> MSSFKYKNSAAGASMQSAANITLRQILEPNNVNLRSKKTHIVCTLGPACKSVETLVKLIDAGMDICRFNFSHGSHEDHKEMFNNVLKAQELRPNCLLGMLLDTKGPEIRTGFLKNKEVHLKEGSKLKLVTDYEFLGDETCIACSYKKLPQSVKPGNIILIADGSVSCKVLETHEDHVITEVLNSAVIGERKNMNLPNVKVDLPIISEKDKNDILNFAIPMGCNFIAASFIQSADDVRLIRNLLGPRGRHIKIIPKIENIEGIIHFDKILAESDGIMIARGDLGMEISPEKVFLAQKLMISKCNLQGKPIITATQMLESMTKNPRPTRAEVTDVANAVLDGTDCVMLSGETAGGKFPVEAVTIMSKICLEAEACIDYKLLYQSLVNAIETPISVQEAVARSAVETAESIQASLIIALTETGYTARLIAKYKPSCTILALSASDSTVKCLNVHRGVTCIKVGSFQGTDIVIRNAIEIAKQRNMAKVGDSVIAIHGIKEEVSGGTNLMKVVQIEL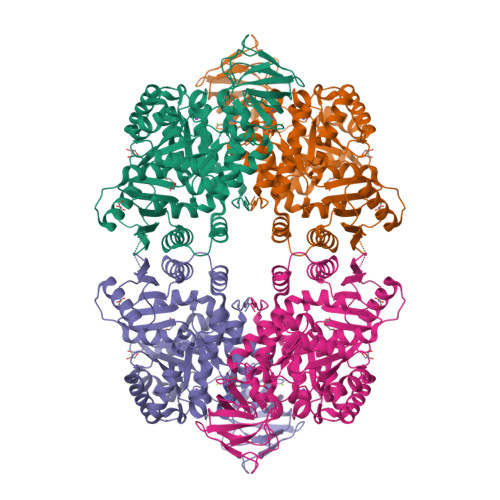EHHHHHH The bacterial RecA, archaeal RadA and eukaryal Rad51 and DMC1 proteins, which belong to a recombinase superfamily, facilitate a central DNA strand-exchange process between a single-stranded DNA (ssDNA) and a homologous double-stranded DNA (dsDNA) in homologous recombination. Archaeal RadAs are close homologues of eukaryal Rad51s (∼40% sequence identity). The structures of EcRecA1 in complex with a series of DNA molecules have shed light on the exact mechanism of homologous DNA-strand exchange. These right-handed helical recombinase assemblies are classic allosteric systems equipped with two functional sites: one located at the subunit interface for binding and hydrolyzing ATP and the other near the filament axis for binding DNA and promoting strand exchange. The series of crystal structures of M. maripaludis RadA presented here further suggest the conservation of an allosteric switch in the ATPase centre which controls the conformational status of DNA-interacting loops.

The second set of MmRadA–AMPPNP structures were determined using crystals in the presence of 0.1–0.4 M NaCl or RbCl or 0.1–0.3 M KCl or NH4Cl. These conditions were selected because they did not appear to provide adequate cationic stabilization to trap the protein in its ATPase-active conformation. Indeed, less ordered structures that were essentially identical to each other were observed. There was no electron density for 19 residues from Ala260 to Val278. In these structures, no plausible ions were seen even for Rb+, which is an electron-rich anomalous scatterer. As such, the catalyzing effect of the monovalent cations seen in the ATPase-active conformation is lost in this second set of MmRadA structures. Compared with the ATPase-active filaments of MmRadA, the filament pitch is slightly longer (108.5 Å). Since very similar filament pitches were observed for multiple data sets under similar ionic conditions (within 0.2 Å), the difference in helical pitches appeared to be significant. ATP hydrolysis would almost certainly lead to the collapse of this stabilizing bridge and result in mobility in loop 2 and hence lower affinity for DNA. Such structural consequences have been observed in the MvRadA–ADP complex, which is essentially similar to the inactive forms observed in the MvRadA–AMPPNP and MmRadA–AMPPNP complexes.

> MADVLTELPGVGPSTADKLIEGGYLDFMKIATATIGELTDIEGISEKAAAKMIMAARDLCDLGFKSGVELLKQRQSVWRLSTGSTELDTVLAGGIESQSVTEFAGMFGSGKTQIMHQTCVNLQMREKIFADLEGVVEEELEAPKAVYIDTEGTFRPERVVQMAEGAGIDGQTVLDNTFVARAYNSDMQMLFAEKIEDLIKGGNNIKLVIIDSLTSTFRNEFTGRGKLAERQQKLGRHMATLNKLADLYNCIVLVTNQVAAKPDAYFGVAEQAIGGHVVGHAATFRFFLRKSKGDKRVAKLYDSPHLPDSEAVFRITEKGIQD1-{3-[6-(tetrahydro-2H-pyran-4-ylamino)imidazo[1,2-b]pyridazin-3-yl]phenyl}ethanone | C19 H20 N4 O2 | 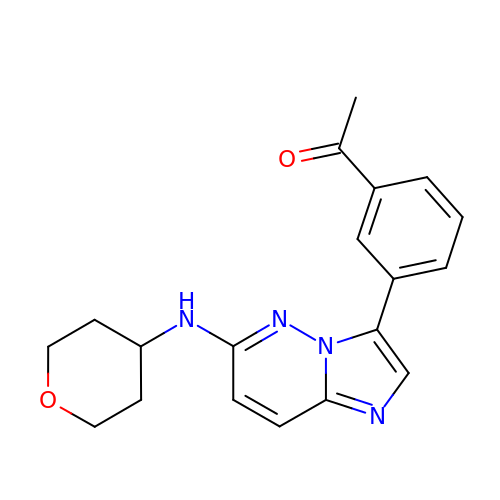DTUZIVBPPQTBFT-UHFFFAOYSA-N ATG9A is the only known ubiquitously expressed transmembrane protein of the autophagy initiation cascade in mammals. The TMD of ATG9A forms an interlocked trimer and functions as a lipid scramblase. The ATG13 and ATG101 subunits of the ULK1 complex form a heteromeric dimer through homologous Hop1/Rev7/Mad2 (HORMA) domains. ATG9A, ATG13, and ATG101 form a multifunctional hub at an early stage of starvation-induced autophagy and mitophagy initiation.

We designed a fusion construct between the HDIR and ATG101, using a flexible linker of five residues (GSDEA) to increase the affinity of the ternary complex for crystallization. We determined the crystal structure of the ATG9A HDIR-ATG101 fusion construct bound to ATG13HORMA to 2.4-Å resolution. The asymmetric unit contains two ATG9A HDIR:ATG13HORMA:ATG101 complexes, both in a similar conformation, except that the ATG101 WF finger is in different conformations in the two complexes due to differences in the crystal packing environment. Our ternary crystal structure of the ATG9A HDIR:ATG13HORMA:ATG101 complex determined that the HDIR binds at the interface between ATG13 and ATG101 HORMA domains. We term the interacting portion of the extreme carboxyl-terminal part of the ATG9A tail the “HORMA dimer–interacting region” (HDIR). This structure shows that the HDIR binds to the HORMA domain of ATG101 by β sheet complementation such that the ATG9A tail resides in a deep cleft at the ATG13:ATG101 interface. The HDIR peptide binds across both HORMA domains within a long hydrophobic groove. ATG101 β2′ (Y45) and ATG13 αA (K15, F16, K18, and F19), αA-B connector (W50), and αC (Y115 and Y118) form a hydrophobic patch of residues, which support the full length of the HDIR. The loop between β2′ and αB in ATG13HORMA (T46-W50) is positioned to support the binding of the HDIR. This rearrangement supports a hydrogen bonding interaction between ATG9A L832 and Q835 and ATG13 K15 and G47. The loop region of G43-Y45 in ATG101 joins a β sheet network between β2 and HDIR residues H837-V839. The interaction between the ATG9A HDIR and ATG13:ATG101 is distal to and thus apparently independent of the safety belt region.

>[4x]GGTSEDELPPQVHKVGSDEAMNCRSEVLEVSVEGRQVEEAMLAVLHTVLLHRSTGKFHYKKEGTYSIGTVGTQDVDCDFIDFTYVRVSSEELDRALRKVVGEFKDALRNSGGDGLGQMSLEFYQKKKSRWPFSDECIPWEVWTVKVHVVALATEQERQICREKVGEKLCEKIINIVEVMNRHEYLPKMPTQSEVDNVFDTGLRDVQPYLYKISFQITD;>[2x]METDLNSQDRKDLDKFIKFFALKTVQVIVQARLGEKICTRSSSSPTGSDWFNLAIKDIPEVTHEAKKALAGQLPAVGRSMCVEISLKTSEGDSMELEIWCLEMNEKCDKEIKVSYTVYNRLSLLLKSLLAITRVTPAYRLSRKQGHEYVILYRIYFGEVQLSGLGEGFQTVRVGTVGTPVGTITLSCAYRINLAFMS Two host-guest collagen peptides (GPP)4-(GXY)4-(GPP)3, where (GXY)4 sequences are from the α1 and α2 chains of human type I collagen, were recombinantly linked to chains A, B and C (corresponding to α1, α2 and α3 in collagen nomenclature and omitted here to avoid confusion) of the NC2 domain in the following combinations designated as α1Aα1Bα1C (for short 111), α1Aα1Bα2C (112), α1Aα2Bα1C (121), α2Aα1Bα1C (211) and α2Aα2Bα2C (222). Three unique chains form a parallel α-helical right-handed bundle. The most important observation is that the triple-helical chain stagger is entirely determined by the NC2 domain.

All five constructs were screened for crystallization, but only three of them yielded crystals of sufficient quality, crystal structures for 111, 211 and 121 were independently solved using the MAD phasing from selenomethionine derivatives (thereafter designated as 111sm, 211sm and 121sm) to 2.25 Å, 2.10 Å and 1.6 Å, respectively. Whereas the crystal packing for 111sm and 211sm are similar (two trimers per asymmetric unit), it differs from that for 121nat or 121sm (one trimer per asymmetric unit). Namely, a triple helical chain linked to chain B of the NC2 domain is always in the leading position, the one linked to A is in the middle, and the third one linked to C is in the trailing position. We suggest here to use a rule of BAC-translation: chain B is leading, A is middle, C is trailing. This way, construct 121 (or α1Aα2Bα1 C) translates into staggering order of α2α1α1, whereas 211 translates into α1α2α1. Despite the variations of composition (homo-trimeric for 111) and stagger (121 or 211) that might not represent a native stagger, the regions of sequences derived from type I collagen are well structured. Crystal structures of 111, 121 and 211 constructs demonstrated that a staggering order can be manipulated at least for short native collagenous sequences, meaning that such sequences are rather adaptive to various abnormal conformations.

>GSGPPGPPGPPGPPGARGEPGNIGFPGPPGPPGPPGRAPTDQHIKQVCMRVIQEHFAEMAASLKRPDSGAT[2x];>[2x]GSGPPGPPGPPGPPGARGQAGVMGFPGPPGPPGPPGRDATDQHIVDVALKMLQEQLAEVAVSAKREALGAV;>GSGPPGPPGPPGPPGARGQAGVMGFPGPPGPPGPPGKEASEQRIRELCGGMISEQIAQLAAHLRKPLAPGSI[2x]>[2x]MMEQVCDVFDIYAICVCCKVESKNEGKKNEVFNNYTFRGLGNKGVLPWKCNSLDMKYFCAVTTYVNESKYEKLKYKRCKYLNKETVDNVNDMPNSKKLQNVVVMGRTTWESIPKKFKPLSNRINVILSRTLKKEDFDEDVYIINKVEDLIVLLGKLNYYKCFIIGGSVVYQEFLEKKLIKKIYFTRINSTYECDVFFPEINENEYQIISVSDVYTSNNTTLDFIIYKKTNNKMLNEQNCIKGEEKNNDMPLKNDDKDTCHMKKLTEFYKNVDKYKINYENDDDDEEEDDFVYFNFNKEKEEKNKNSIHPNDFQIYNSLKYKYHPEYQYLNIIYDIMMNGNKQSDRTGVGVLSKFGYIMKFDLSQYFPLLTTKKLFLRGIIEEL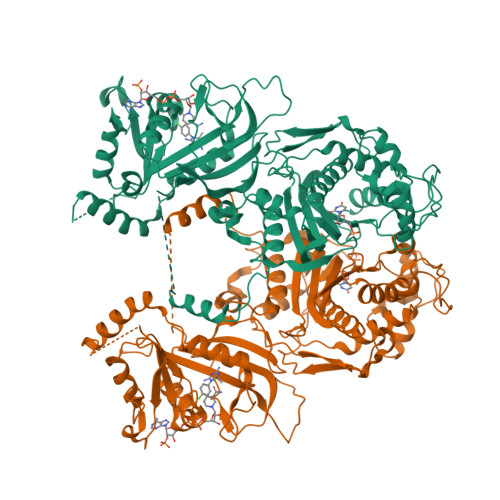LWFIRGETNGNTLLNKNVRIWEANGTREFLDNRKLFHREVNDLGPIYGFQWRHFGAEYTNMYDNYENKGVDQLKNIINLIKNDPTSRRILLCAWNVKDLDQMALPPCHILCQFYVFDGKLSCIMYQRSCDLGLGVPFNIASYSIFTHMIAQVCNLQPAQFIHVLGNAHVYNNHIDSLKIQLNRIPYPFPTLKLNPDIKNIEDFTISDFTIQNYVHHEKISMDMAA> FTLIELMIVVAIIGILAAIAIPQYQNYVARSEG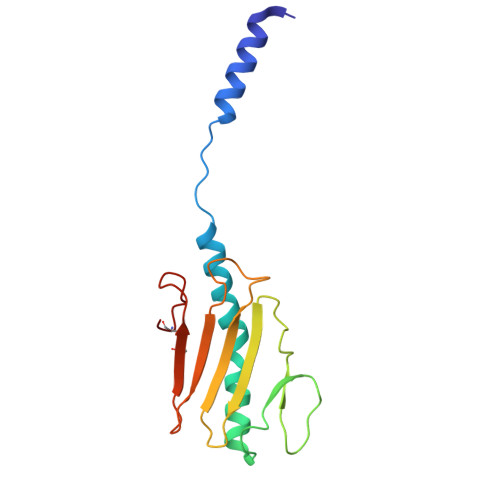ASALATINPLKTTVEESLSRGIAGSKIKIGTTASTATETYVGVEPDANKLGVIAVAIEDSGAGDITFTFQTGTSSPKNATKVITLNRTADGVWACKSTQDPMFTPKGCDN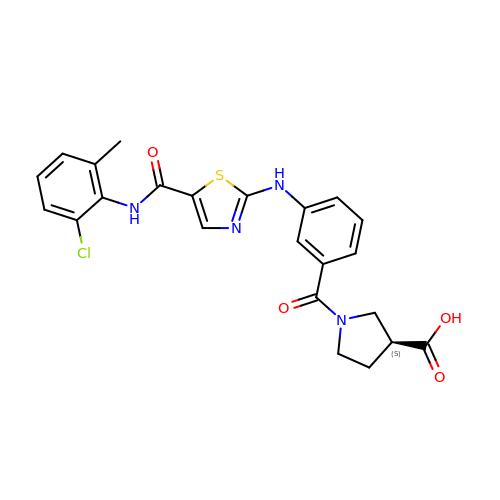(3~{S})-1-[3-[[5-[(2-chloranyl-6-methyl-phenyl)carbamoyl]-1,3-thiazol-2-yl]amino]phenyl]carbonylpyrrolidine-3-carboxylic acid | C23 H21 Cl N4 O4 S | RQFQWAHQNYFCJN-HNNXBMFYSA-N>[2x]QSACTLQSETHPPLTWQKCSSGGTCTQQTGSVVIDANWRWTHATNSSTNCYDGNTWSSTLCPDNETCAKNCCLDGAAYASTYGVTTSGNSLSIDFVTQSAQKNVGARLYLMASDTTYQEFTLLGNEFSFDVDVSQLPCGLNGALYFVSMDADGGVSKYPTNTAGAKYGTGYCDSQCPRDLKFINGQANVEGWEPSSNNANTGIGGHGSCCSEMDIWEANSISEALT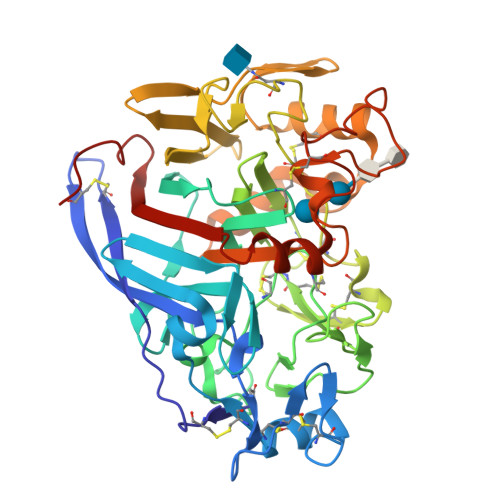PHPCTTVGQEICEGDGCGGGTCDPDGCDWNPYRLGNTSFYGPGSSFTLDTTKKLTVVTQFETSGAINRYYVQNGVTFQQPNAELGSYSGNELNDDYCTAEEAEFGGSSFSDKGGLTQFKKATSGGMVLVMSLWDDYYANMLWLDSTYPTNETSSTPGAVRGSCSTSSGVPAQVESQSPNAKVTFSNIKFGPIGSTGNPSG>DRHHHHHHKLVPGTPPLFNVSLDVAPEQRWLPMLRHYDPDFLRTAVAQVIGDRVPQWVLGMVGEIVSKVESFL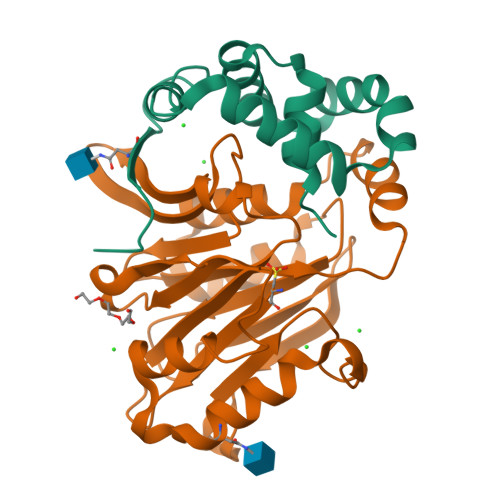PQPFTDEIRSICDSLSLSLADGILVNLAYEASAF[2x];>[2x]CTSIVAQDSQGRIYHGRNLDYPFGKILRKLTADVQFIKNGQIAFTGTTFVGYVGLWTGQSPHKFTISGDERDKGWWWENMIAALSLGHSPISWLIRKTLSESESFEAAVYTLAKTPLIADVYYIVGGTSPKEGVVITRDRGGPADIWPLDPLNGEWFRVETNYDHWKPAPKVDDRRTPAIKALNATGQAHLNLETLFQVLSLFPVYNSYTIYTTVMSAAEPDKYLTMIRNPS> MASSRSELLLDRFAEKIGVGSISFNENRLCSFAIDEIYYISLSDANDEYMMIYGVCGKFPTDNPNFALEILNANLWFAENGGPYLCYESGAQSLLLALRFPLDDATPEKLENEIEVVVKSMENLYLVLHNQGITLENEH;> MGSSHHHHHHSQDPGGTGHLISSTGALGSRSLFSPLRNSMADSVDSRDIPGLPTNPSRLAAAT

Enteropathogenic Escherichia coli injects effector proteins into host cells using a type III secretion system (T3SS). The translocated intimin receptor (Tir) is the first effector delivered into host cells and imparts efficient secretion of other effectors. However, it was later reclassified as a multi-cargo chaperone because it interacts with at least 9 other effectors, most of which require CesT for translocation into host cells. We provide evidence that the multi-cargo chaperone CesT binds to two regions in Tir at the N- and C-terminus through a specific recognition motif, and show that CesT binding to the Tir C-terminus is important for host translocation.

Here, we present the co-crystal structure of a C-terminal truncation of CesT in complex with an N-terminal fragment of Tir. The Tir32-80-CesT138 complex produced crystals in the trigonal space-group P322 with one molecule of the complex in the asymmetric unit. Diffraction data were collected to 2.74 Å resolution and the structure was determined by molecular replacement. Residues 130–138 of CesT138, the N-terminal histidine tag, and residues 32–34, 54–64, and 76–80 of Tir were not included in the final model due to poor or absent electron density. Tir residues 35–53 adopt a β-hairpin-like fold and extend the 5-stranded β-sheet core of CesT138, while also being pinched between α1 and orthogonally below by α3 of CesT138. Tir residues 65–75 are bound along the concave surface of the β-sheet core of CesT138. Specifically, Tir residues I38 (purple), L44 (cyan), and L49 (cyan) anchor the β-hairpin-like peptide to CesT138; and L69 plus three additional proline residues make a second point of contact with the β-sheet core of CesT138. Although only one molecule of CesT138 was present in the crystallographic asymmetric unit, the dimer interface is clearly present along the principle 2-fold axis of symmetry. Interestingly, the CesT C-terminus occupies the same binding surface as Tir residues 65–75 (pink), despite significantly different sequences. Taken together, the structural data from the Tir32-80-CesT138 and CsrA-CesT complexes suggest that (i) CesT exists as an unswapped dimer, (ii) the Tir binding region of CesT exhibits significant plasticity that could accommodate the binding of multiple effectors with varying sequences, and (iii) the C-terminal extension of CesT is required for CsrA interaction that in turn could also prevent CesT from binding Tir.>MHHHHHHAMGEGVEITFNVNDYDNTLTVYTTRPDTFMGCTYLAVAAGHPLAQKAAENNPELAAFIDECRNTKVAEAEMATMEKKGVDTGFKAVHPLTGEEIPVWAANFVLMEYGTGAVMAVPGHDQR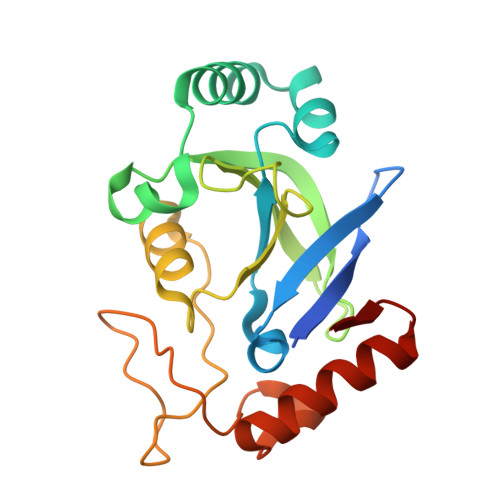DYEFASKYGLNIKPVILAADGSEPDLSQQALTEKGVLFNSGEFNGLDHEAAFNAIADKLTAMGVGERKV[2x]>[2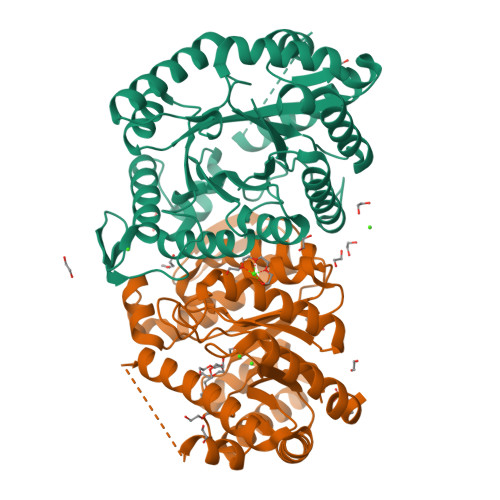x]MKFGINLFPTVGPAEKSAGQHFEESLRLAELADELGFHHVKTVEHYFHEYGGYSPDPVTFLAAAAARTRRVRLVTGAVLPVFTHPLKLAGKLAMLDNISQGRLDVGFGRAFLPDEFTAFEISMDESRARFDEGVEAVRRLWAEEDVVWEGTFHRFGPVTMLPRTWQRPHPRILVATAKTPASAEAAARAGHGVMLVPSINPREQVQKTLSLYRDAASAAGFKPTEEDIHMSYNCYLAEDGQEARQKGGQASERANRALASAVSAWRETRSADYPGYEKIVEKAGRGDFDRAVAERKALVGTPDEVRAAIDDIRGWFGDFTISLQVISGAMPFEESARTMRLFAEHLLPHYAAND>[3x]GHPETLVKVKDAEDQLGARVGYIELDLNSGKILESFRPEERFPMMSTFKVLLCGAVLSRVDAGQEQLGRRIHYSQNDLVEYSPVTEKHLTDGMTVRELCSAAITMSDNTAANLLLTTIGGPKELTAFLHNMGDHVTRLDRWEPELNEAIPNDERDTTTPAAMATTLRKLLTGELLTLASRQQLIDWMEADKVAGPLLRSALPAGWFIADKSGAGERGSRGIIAA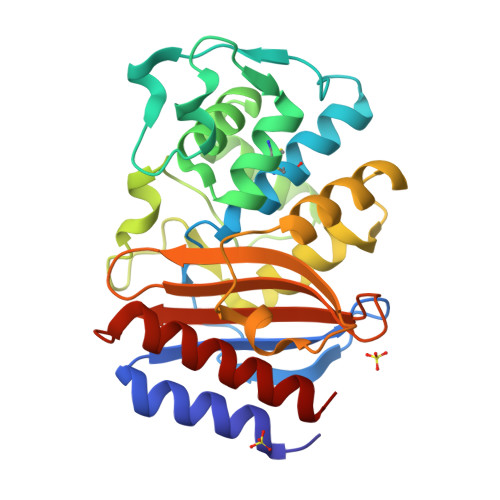LGPDGKPSRIVVIYTTGSQATMDERNRQIAEIGASLIKHW NTA is catalyzed by a group of enzymes called N-terminal acetyltransferases (NATs), which belong to the Gcn5-related N-acetyltransferase (GNAT) family of enzymes. NatA and NatB are heterodimeric complexes, each with a distinctive catalytic subunit (NAA10 in NatA and NAA20 in NatB; Starheim et al., 2008) and a unique auxiliary subunit (NAA15 in NatA and NAA25 in NatB; Arnesen et al., 2005). NatA accounts for 38% of the human N-terminal acetylome, acetylating small N-terminal residues after removal of the initial methionine residue, while NatB modifies N-termini with sequences of MD-, ME-, MN-, and MQ-. In addition, hNatB is upregulated in human hepatocellular carcinoma, where it has been suggested as a potential therapeutic target as silencing of this complex can block cell proliferation and tumor formation. hNatB-mediated NTA of α-synuclein (αSyn) has been shown to increase αSyn stability and lipid binding, and to reduce aggregation capacity.

In this study, we report the 3.5 Å resolution cryo-electron microscopy (cryo-EM) structure of the ~130 KDa hNatB bound to a bisubstrate CoA-αSyn conjugate together with a structure-guided analysis of mutational effects on catalytic activity. Consistent with previous NAT structural studies, the atomic model of hNatB features a catalytic subunit, hNAA20, that adopts a canonical Gcn5-related N-acetyltransferase (GNAT) fold (Deng and Marmorstein, 2020; Neuwald and Landsman, 1997). The 21 helices of the core region also form a number of TPR motifs, which come together to form a ring that completely wraps around and extensively contacts hNAA20 within its hollow center. The α28 helix closes the core ring structure, locking hNAA20 in position, and bridging the N- and C-terminal and regions. While no corresponding small molecules have been identified to play a similar role in hNatB, our model shows that this interaction is replaced by an extended loop that connects the α31 helix with the α32 helix of hNatB-NAA25. In the cryo-EM map, density for the CoA-αSyn conjugate bisubstrate inhibitor is well resolved, allowing us to confidently model the CoA portion and the first 5 N-terminal residues (of 10 residues present) of the αSyn portion. Here we observe that the positively charged hNAA20-Arg85 interacts with the negatively charged 3'-phosphorylated ADP portion of CoA to form a salt bridge while Arg84 makes Van der Waals interactions. Hydrogen bonds are formed between the backbone N-H group of αSyn-Met1 and the backbone carbonyl group of hNAA20-Phe111, as well as the backbone carbonyl group of αSyn-Met1 with the sidechain of hNAA20-Tyr138. The only sidechain that forms a hydrogen bond with hNAA20 is αSyn-Asp2, which hydrogen bonds with a hNAA20-His73 ring nitrogen and the hNAA20-Thr75 sidechain.

> MTTLRAFTCDDLFRFNNINLDPLTETYGIPFYLQYLAHWPEYFIVAEAPGGELMGYIMGKAEGSVAREEWHGHVTALSVAPEFRRLGLAAKLMELLEEISERKGGFFVDLFVRVSNQVAVNMYKQLGYSVYRTVIEYYSASNGEPDEDAYDMRKALSRDTEKK;> MATRGHVQDPNDRRLRPIYDYLDNGNNKMAIQQADKLLKKHKDLHCAKVLKAIGLQRTGKQEEAFTLAQEVAALEPTDDNSLQALTILYREMHRPELVTKLYEAAVKKVPNSEEYHSHLFMAYARVGEYKKMQQAGMALYKIVPKNPYYFWSVMSLIMQSISAQDENLSKTMFLPLAERMVEKMVKEDKIEAEAEVELYYMILERLGKYQEALDVIRGKLGEKLTSEIQSRENKCMAMYKKLSRWPECNALSRRLLLKNSDDWQFYLTYFDSVFRLIEEAWSPPAEGEHSLEGEVHYSAEKAVKFIEDRITEESKSSRHLRGPHLAKLELIRRLRSQGCNDEYKLGDPEELMFQYFKKFGDKPCCFTDLKVFVDLLPATQCTKFINQLLGVVPLSTPTEDKLALPADIRALQQHLCVVQLTRLLGLYHTMDKNQKLSVVRELMLRYQHGLEFGKTCLKTELQFSDYYCLLAVHALIDVWRETGDETTVWQALTLLEEGLTHSPSNAQFKLLLVRIYCMLGAFEPVVDLYSSLDAKHIQHDTIGYLLTRYAESLGQYAAASQSCNFALRFFHSNQKDTSEYIIQAYKYGAFEKIPEFIAFRNRLNNSLHFAQVRTERMLLDLLLEANISTSLAESIKSMNLRPEEDDIPWEDLRDNRDLNVFFSWDPKDRDVSEEHKKLSLEEETLWLRIRSLTLRLISGLPSLNHPVEPKNSEKTAENGVSSRIDILRLLLQQLEATLETGKRFIEKDIQYPFLGPVPTRMGGFFNSGCSQCQISSFYLVNDIYELDTSGLEDTMEIQERIENSFKSLLDQLKDVFSKCKGDLLEVKDGNLKTHPTLLENLVFFVETISVILWVSSYCESVLRPYKLNLQKKKKKKKETSIIMPPVFTSFQDYVTGLQTLISNVVDHIKGLETHLIALKLEELILEDTSLSPEERKFSKTVQGKVQSSYLHSLLEMGELLKKRLETTKKLKI;> MDVFM> MRQTLPCIYFWGGLLPFGMLCASSTTKCTVSHEVADCSHLKLTQVPDDLPTNITVLNLTHNQLRRLPAANFTRYSQLTSLDVGFNTISKLEPELCQKLPMLKVLNLQHNELSQLSDKTFAFCTNLTELHLMSNSIQKIKNNPFVKQKNLITLDLSHNGLSSTKLGTQVQLENLQELLLSNNKIQALKSEELDIFANSSLKKLELSSNQIKEFSP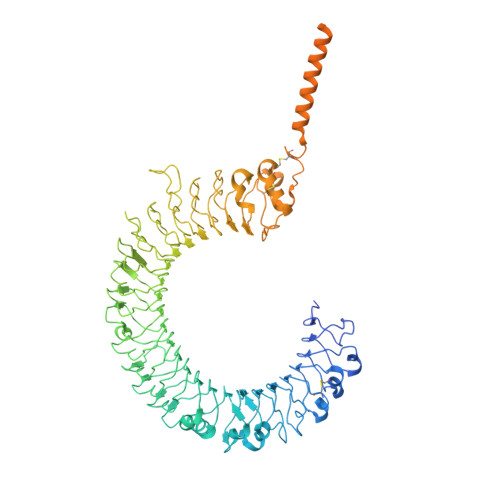GCFHAIGRLFGLFLNNVQLGPSLTEKLCLELANTSIRNLSLSNSQLSTTSNTTFLGLKWTNLTMLDLSYNNLNVVGNDSFAWLPQLEYFFLEYNNIQHLFSHSLHGLFNVRYLNLKRSFTKQSISLASLPKIDDFSFQWLKCLEHLNMEDNDIPGIKSNMFTGLINLKYLSLSNSFTSLRTLTNETFVSLAHSPLHILNLTKNKISKIESDAFSWLGHLEVLDLGLNEIGQELTGQEWRGLENIFEIYLSYNKYLQLTRNSFALVPSLQRLMLRRVALKNVDSSPSPFQPLRNLTILDLSNNNIANINDDMLEGLEKLEILDLQHNNLARLWKHANPGGPIYFLKGLSHLHILNLESNGFDEIPVEVFKDLFELKIIDLGLNNLNTLPASVFNNQVSLKSLNLQKNLITSVEKKVFGPAFRNLTELDMRFNPFDCTCESIAWFVNWINETHTNIPELSSHYLCNTPPHYHGFPVRLFDTSSCKDSAPFELFFMINTSILLIFIFIVLLIHFEGWRISFYWNVSVHRVLGFKEIDRQTEQFEYAAYIIHAYKDKDWVWEHFSSMEKEDQSLKFCLEERDFEAGVFELEAIVNSIKRSRKIIFVITHHLLKDPLCKRFKVHHAVQQAIEQNLDSIILVFLEEIPDYKLNHALCLRRGMFKSHCILNWPVQKERIGAFRHKLQVALGSKNSVH>TDKLTSLRQYTTVVAATGDIAAMKLYQPQDATTNPSLI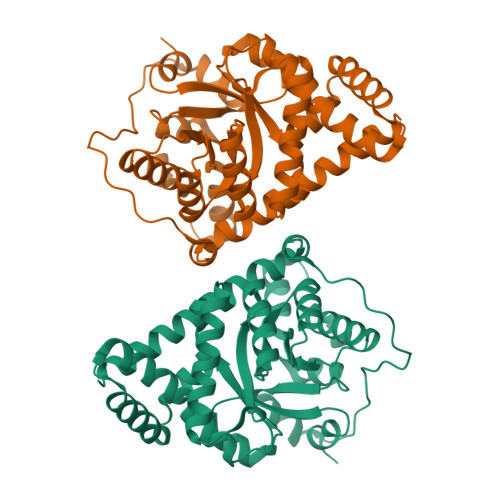LNAAQIPEYRKLIDDAVAWAKQQSNDRAQQIVDATDKLAVNIGLEILKLVPGRISTEVDARLSYDTEASIAKAKRLIKLYNDAGISNDRILIKLASTWQGIRAAEQLEKEGINCNLTLLFSFAQARACAEAGVFLISPFVGRILDWYKANTDKKEYAPAEDPGVVSVSEIYQYYKEHGYETVVMGASFRNIGEILELAGCDRLTIAPALLKELAESEGAIERKLSYTGEVKARPARITESEFLWQHNQDPMAVDKLAEGIRKFAIDQEKLEKMIGDLL[2x]> MAVPFVEDWDLVQTLGEGAYGEVQLAVNRVTEEAVAVKIVDMKRAVDCPENIKKEICINKMLNHENVVKFYGHRREGNIQYLFLEYCSGGELFDRIEPDIGMPEPDAQRFFHQLMAGVVYLHGIGITHRDIKPENLLLDERDNLKISDFGLATVF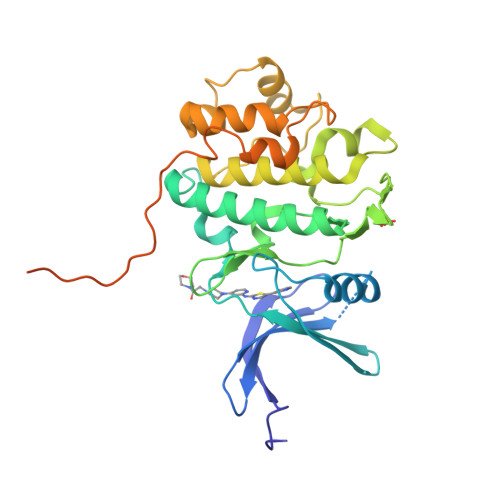RYNNRERLLNKMCGTLPYVAPELLKRREFHAEPVDVWSCGIVLTAMLAGELPWDQPSDSCQEYSDWKEKKTYLNPWKKIDSAPLALLHKILVENPSARITIPDIKKDRWYNKPLKKGAKRPRVTSGGVSESPSGFSKHIQSNLDFSPVNSASRTPGSGWSKEHHHHHH> STKFSDNYDVKEELGKGAFSVVRRCVHKTTGLEFAAKIINTKKLSARDFQKLEREARICRKLQHPNI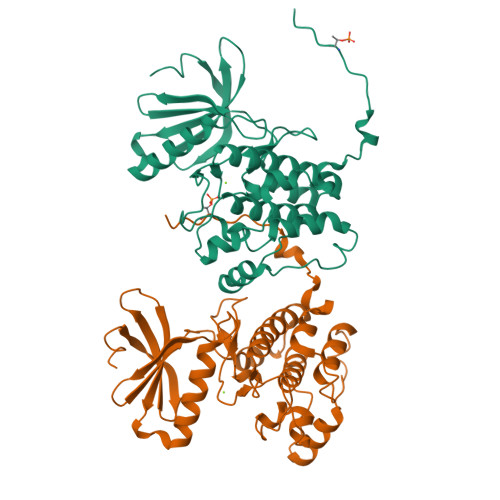VRLHDSIQEESFHYLVFDLVTGGELFEDIVAREFYSEADASHCIQQILESIAYCHSNGIVHRNLKPENLLLASKAKGAAVKLADFGLAIEVNDSEAWHGFAGTPGYLSPEVLKKDPYSKPVDIWACGVILYILLVGYPPFWDEDQHRLYAQIKAGAYDYPSPEWDTVTPEAKSLIDSMLTVNPKKRITADQALKVPWICNRERVASAIHRQDTVDCL> GPMPKPINVRVTTMDAELEFAIQPNTTGKQLFDQVV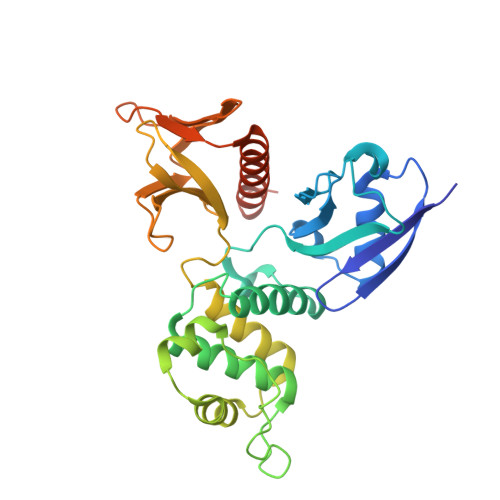KTVGLREVWFFGLQYVDSKGYSTWLKLNKKVTQQDVKKENPLQFKFRAKFFPEDVSEELIQEITQRLFFLQVKEAILNDEIYCPPETAVLLASYAVQAKYGDYNKEIHKPGYLANDRLLPQRVLEQHKLTKEQWEERIQNWHEEHRGMLREDSMMEYLKIAQDLEMYGVNYFEIKNKKGTELWLGVDALGLNIYEHDDKLTPKIGFPWSEIRNISFNDKKFVIKPIDKKAPDFVFYAPRLRINKRILALCMGNHELYMRRRKPDTIEVQQMKAQAR> GSHMARAQVSEAILLAEGQKSAVTEYYLNHGEWPGDNS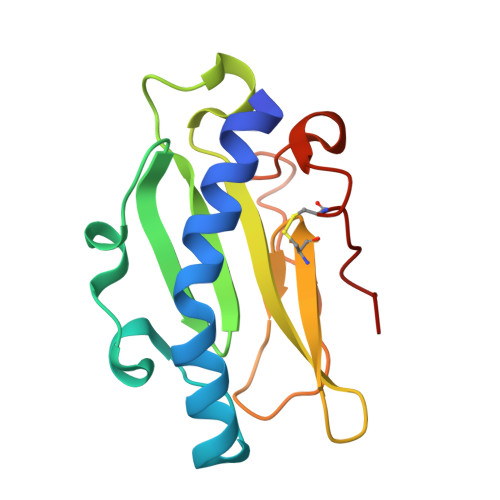SAGVATSADIKGKYVQSVTVANGVITAQMASSNVNNEIKSKKLSLWAKRQNGSVKWFCGQPVTRTTATATDVAAANGKTDDKINTKHLPSTCRDDSSAS> DGLNGTMMQYYEWHLENDGQHWNRLHDDAAALSDAGITAIWIPPAYKGNSQADVGYGAYDLYDLGEFNQKGTVRTKYGTKAQLERAIGSLKSNDINVYGDVVMNHKMGADFTEAVQAVQVNPTNRWQDISGAYTIDAWTGF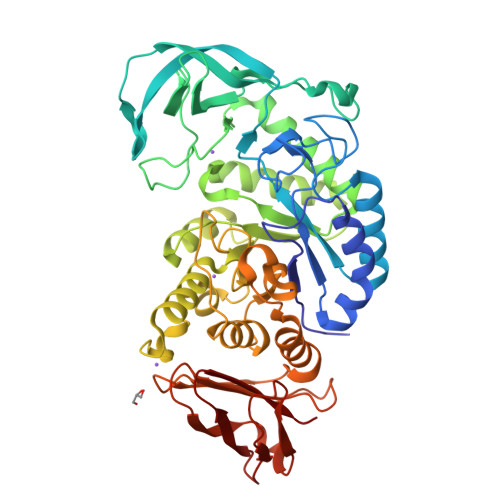DFSGRNNAYSDFKWRWFHFNGVDWDQRYQENHIFRFANTNWNWRVDEENGNYDYLLGSNIDFSHPEVQDELKDWGSWFTDELDLDGYRLDAIKHIPFWYTSDWVRHQRNEADQDLFVVGEYWKDDVGALEFYLDEMNWEMSLFDVPLNYNFYRASQQGGSYDMRNILRGSLVEAHPMHAVTFVDNHDTQPGESLESWVADWFKPLAYATILTREGGYPNVFYGDYYGIPNDNISAKKDMIDELLDARQNYAYGTQHDYFDHWDVVGWTREGSSSRPNSGLATIMSNGPGGSKWMYVGRQNAGQTWTDLTGNNGASVTINGDGWGEFFTNGGSVSVYVNQ The physiologically important protein PGM1 is an evolutionary conserved enzyme that belongs to the ubiquitous and ancient α-d-phosphohexomutase superfamily, and it is encoded by the PGM1 gene. PGM1 is a key regulator of carbohydrate metabolism in mammalian cells, catalyzing the reversible conversion between α-d-glucose 1-phosphate (G1P) and α-d-glucose 6-phosphate (G6P) via a bisphosphorylated sugar intermediate, α-d-glucose 1,6-bisphoshate (G16P). Isoform 2 of human PGM1 encodes a protein comprising 580 residues, and it differs from isoform 1 by having a longer and different N-terminal. Here we present three crystal structures of the isoform 2 variant of PGM1, both as a free enzyme and in complex with substrate and product.

We here publish, for the first time, data for a eukaryotic PGM that show the detailed structures of both the pre- and post-reaction complexes. Finally, the complex structures have strong densities for G1P and G6P in their active sites. The metal ions in the two complex crystal structures are most likely Zn2+, due to the crystallization and soaking conditions (see Experimental procedures), rather than Mg2+ that is required for enzymatic activity, explaining the stability of substrate and product complexes for structural studies. The divalent cations in the active sites are in both structures complexed by three conserved Asp residues (Asp306, Asp308, and Asp310) contributed by the D2 metal-binding loop. Only minor differences can be seen when comparing the free protein structure with the complex structures, with D4 rotated 2° or less in the complexes, compared to the free protein structure.

> GAMGSDFEEWISGTYRKMEEGPLPLLTFATAPYHDQKPGTSGLRKKTYYFEEKPCYLENFIQSIFFSIDLKDRQGSSLVVGGDGRYFNKSAIETIVQMAAANGIGRLVIGQNGILSTPAVSCIIRKIKAIGGIILTASHNPGGPNGDFGIKFNISNGGPAPEAITDKIFQISKTIEEYAVCPDLKVDLGVLGKQQFDLENKFKPFTVEIVDSVEAYATMLRSIFDFSALKELLSGPNRLKIRIDAMHGVVGPYVKKILCEELGAPANSAVNCVPLEDFGGHHPDPNLTYAADLVETMKSGEHDFGAAFDGDGDRNMILGKHGFFVNPSDSVAVIAANIFSIPYFQQTGVRGFARSMPTSGALDRVASATKIALYETPTGWKFFGNLMDASKLSLCGEESFGTGSDHIREKDGLWAVLAWLSILATRKQSVEDILKDHWQKYGRNFFTRYDYEEVEAEGANKMMKDLEALMFDRSFVGKQFSANDKVYTVEKADNFEYSDPVDGSISRNQGLRLIFTDGSRIVFRLSGTGSAGATIRLYIDSYEKDVAKINQDPQVMLAPLISIALKVSQLQERTGRTAPTVIT>[2x]MAFAKELFLGKIKKKEVFPFPEVSQDELNEINQFLGPVEKFFTEEVDSRKIDQEGKIPDETLEKLKSLGLFGLQVPEEYGGLGFSNTMY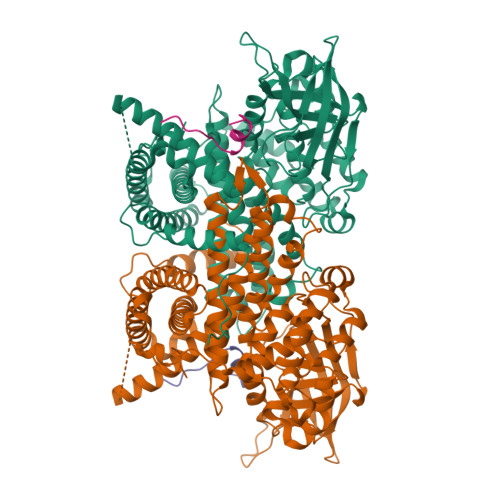SRLGEIISMDGSITVTLAAHQAIGLKGIILAGTEEQKAKYLPKLASGEHIAAFCLTEPASGSDAASIRSRATLSEDKKHYILNGSKVWITNGGLANIFTVFAKTEVVDSDGSVKDKITAFIVERDFGGVTNGKPEDKLGIRGSNTCEVHFENTKIPVENILGEVGDGFKVAMNILNSGRFSMGSVVAGLLKRLIEMTAEYACTRKQFNKRLSEFGLIQEKFALMAQKAYVMESMTYLTAGMLDQPGFPDCSIEAAMVKVFSSEAAWQCVSEALQILGGLGYTRDYPYERILRDTRILLIFEGTNEILRMYIALTGLQHAGRILTTRIHELKQAKVSTVMDTVGRRLRDSLGRTVDLGLTGNHGVVHPSLADSANKFEENTYCFGRTVETLLLRFGKTIMEEQLVLKRVANILINLYGMTAVLSRASRSIRIGLRNHDHEVLLANTFCVEAYLQNLFSLSQLDKYAPENLDEQIKKVSQQILEKRAYICAHPLDRTCHHHHHH;>[2x]MGQDPVELAMFGLRHMEPDLSARVTIYQVPLPKDSTGAADPPQPHIVGIQSPDQQAALARHNPARPVFVEGPFSLWLRNKCVYYHILRADLLPPEEREVEETPEEWNLYYPMQLDLEYVRSGWDNYEFDINEVEEGPVFAMCMAGAHDQATMAKWIQGLQETNPTLAQIPVVFRLAGSTRELQTSSAGLEEPPLPEDHQEEDDNLQRQQQGQSLEHHHHHH>[2x]DQ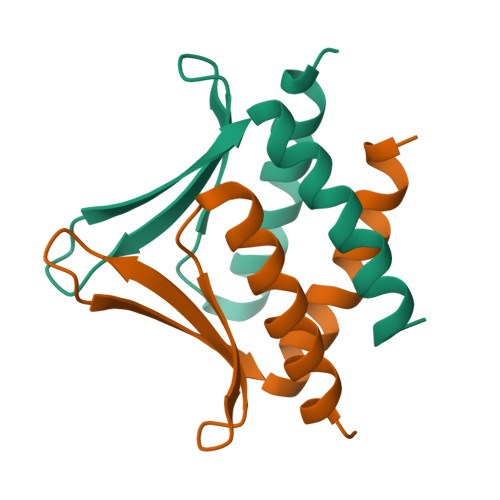YKPKLELLSERLNEEMKRIGTDINFSYNDTIKGLVVSVKDANGDKVIREIPSKEAVELMQRMRDVIGIIFD N-[(furan-2-yl)methyl]-2-phenylquinazolin-4-amine 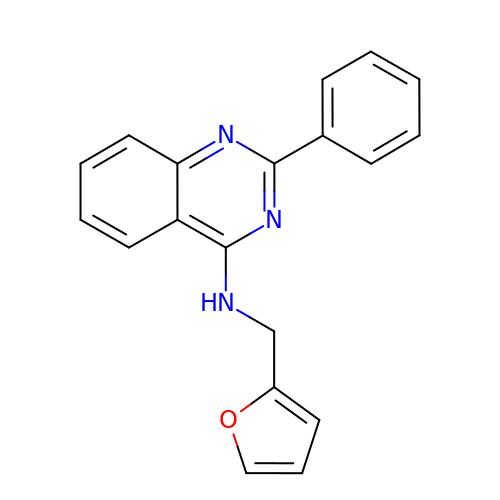| C19 H15 N3 O | AZNLVBWSZDPKAA-UHFFFAOYSA-N>MTTTTTKKPHVLVIPFPQSGHMVPHLDLTHQILLRGATVTVLVTPKNSSYLDALRSLHSPEHFKTLILPFPSHPCIPSGVESLQQLPLEAIVHMFDALSRLHDPLVDFLSRQPPSDLPDAILGSSFLSPWINKVADAFSIKSISFLPINAHSISVMWAQEDRSFFNDLETATTESYGLVINSFYDLEPEFVETVKTRFLNHHRIWTVGPLLPFKAGVDRGGQSSIPPAKVSAWLDSCPEDNSVVYVGFGSQIRLTAEQ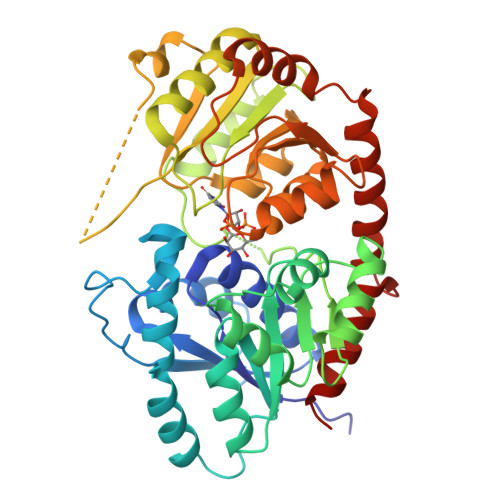TAALAAALEKSSVRFIWAVRDAAKKVNSSDNSVEEDVIPAGFEERVKEKGLVIRGWAPQTMILEHRAVGSYLTHLGWGSVLEGMVGGVMLLAWPMQADHFFNTTLIVDKLRAAVRVGENRDSVPDSDKLARILAESAREDLPERVTLMKLREKAMEAIKEGGSSYKNLDELVAEMCL[4x]>[6x]MEKFQILALSGGGYRGLFTATVLKELEQEAKENGHDSIADCFDLITGTSVGGIVALAIAYGIKVEAIVDLFKSHGDKIFQPKPFLKFTGSKYSNESLKTVLEEWFGDSILGDLKCPVVIPTIDFT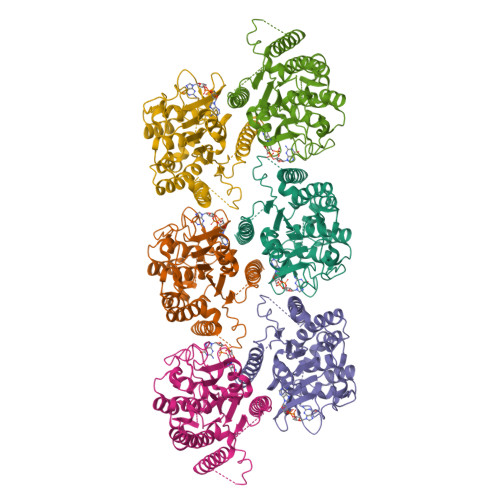RGSPVTLKTPHNPNLKRDWKLKIVDVALATSAAPTYFPRHPIGPNEYVAGGLFANDPSLIGLHEADYMFKKNIQDVHILSIGTLSSKKQLNPSTKKDGGYLDWGEGSILKAAPNIIDLVLSSQQQFMEQMVKHRMEPFPNQFYKIDEQIVQASAQFIGLDETSDAAKQVLEGNGIQSAKVALGKDFIRNYFNQPSRKREWFDGPQKNV> NPVENYIDSVLNEVLVVPNIQPSTSVSSHAAPALDAAETGHTSSVQPEDMIETRYVITDQTRDETSIESFLGRSGCIAMIEFNTSSDKTEHDKIGKGFKTWKVSLQEMAQIRRKYELFTYTRFDSEITIVTAAAAQGNDSGHIVLQFMYVPPGAPVPEKRDDYTWQSGTNASVFWQEGQPYPRFTIPFMSIASAYYMFYDGYDGDSAASKYGSVVTNDMGTICVRIVTSNQKHDSNIVCRIYHKAKHIKAWCPRPPRAVAYQHTHSTN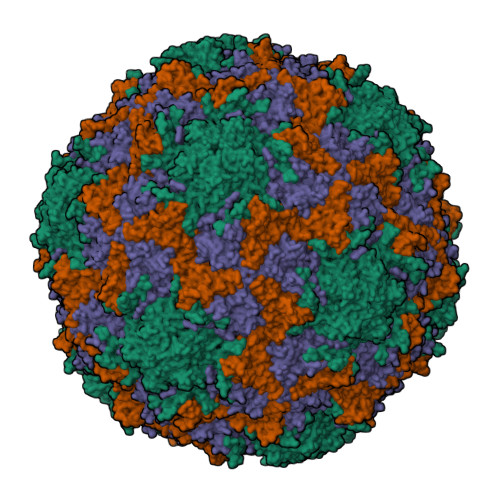YIPSNGEATTQIKTRPD;> SDRLIQITRGDSTITSQDTANAVVAYGVWPSYLTPDDATAIDKPTQPDTSSNRFYTLDSRSWTSASSGWWWKLPDALKNMGIFGENMFYHFLGRSGYTIHVQCNSSKFHQGLLIVAAIPEHQLASATSGNVSVGYNHTHPGEQGREVVPSRTSSDNKRPSDDSWLNFDGTLLGNLPIYPHQYINLRTNNSATLILPYVNAVPMDSMLRHNNWSLVIIPICPLQVQPGGTQSIPITVSISPMFSEFSGPRSKVVF;> SPSAFPYFHPTKEIFIPGQVRNLIEMCQVDTLIPVNNTQENVRSVNMYTVDLRTQVDLAKEVFSIPVDIASQPLATTLIGELASYYTHWTGSLRFSFMFCGSASSTLKLLIAYTPPGVGKPKSRREAMLGTHLVWDVGLQSTASLVVPWVSASHFRFTTPDTYSSAGYITCWYQTNFVVPDSTPDNAKMVCMVSACKDFCLRLARDTNLHTQEG;> NINYFKDAASSGASRLD>ATKKAVAVLKGNSNVEGVVTLSQDDDGPTTVNVRITGLAPGLHGFHLHEYGDTTNGCMSTGAHFNPNKLTH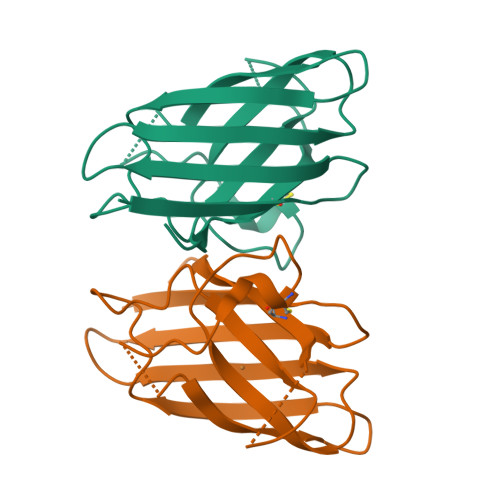GAPGDEIRHAGDLGNIVANADGVAEVTLVDNQIPLTGPNSVVGRALVVHELEDDLGKGGHELSLTTGNAGGRLACGVVGLTPI[8x]> MLSYFQGFVPIHTIFYSVFHPTEGSKIKYEFPPNNLKNHGINFNTFKNYIIPKPILCHKLITFKYGTYRIVCYPVTINSPIYARNFFSFNFVFVFPYDCETSPYEPAITRLGKMFKVLEEQNQLLSKSERDPVFFDLKVLENSTTTPSTAGPSSTPNPSSNTTPTHPTSEKDTKDMRSSRYSDLIKDLGLPQSAFSIQDLLMRIFQDLNNYS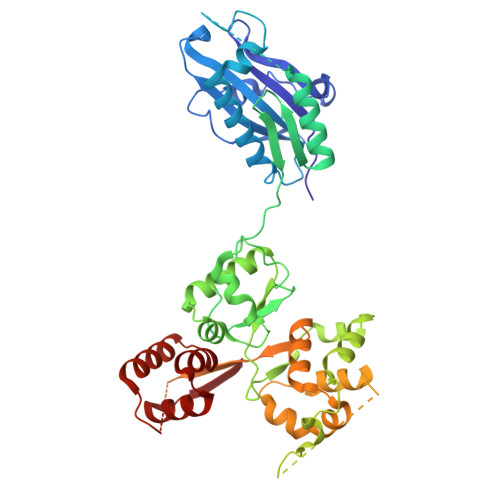ECLIPIDEGNAVDIKIFPLLRPPTTCVSLEDVPLSSVNLKKIIDVNWDPTMMSIVPYIDGLNSIAKISKLSNSDPGLVIECIRHLIYYKCVTLSDIFQFSNIYAPSSLIRNFLTDPLMASDCQSYVTFPEVSKISNLPLNKSLGSGDQDSPSFSVRRKSKSSSIPSNPDSRTTSFSSTSRVSQNSSLNSSFSSIYKDWRQSQTSCSSSNIHVINNRNRFLPTRSCLFDLYRSLSQGQTLKTWYESKYMILKENNIDIRRFITFGLEKRIIYRCYSFPVMINAGSREPKEMTPIITKDLVNNDKLLEKRNHNHLLSATGSRNTAQSGNLKPERPSKVSFEMQRVSSLATGKSTMPKLSDEEEGILEESIRNAETFDKICVLLSKPKLEVESYLNELGEFKVINS>[12x]MGRILDISGQPFDFDDEMQSRSDELAMVMKRTQEHPSSGVTPNRAAQMLRDAERGDLTAQADLAFDMEEKDTHLFSELSKRRLAIQALEWRIAPARDASAQEKKDADMLNEYLHDAAWFEDALFDAGDAILKGYSMQEIEWGWLGKMRVPVALHHRDPALFCANPDNLNELRLRDASYHGLELQPFGWFMHRAKSRTGYVGTNGLVRTLIWPFIFKNYSVRDFAEFLEIYGLPMRVGKYPTGSTNREKATLMQAVMDIGRRAGGIIPMGMTLDFQSAADGQSDPFMAMIGWAEKAISKAILGGTLTTEAGDKGARSLGEVHDEVRREIRNADVGQLARSINRDLIYPLLALNSDSTIDINRLPGIVFDTSEAGDITALSDAIPKLAAGMRIPVSWIQEKLHIPQPVGDEAVFTIQPVVPDNGSQKEAALSAEDIPQEDDIDRMGVSPEDWQRSVDPLLKPVIFSVLKDGPEAAMNKAASLYPQMDDAELIDMLTRAIFVADIWGRLDAAADH;>[12x]MNYATVNDLCARYTRTRLDILTRPKTADGQPDDAVAEQALADASAFIDGYLAARFVLPLTVVPSLLKRQCCVVAWFYLNESQPTEQITATYRDTVRWLEQVRDGKTDPGVESRTAASPEGEDLVQVQSDPPVFSRKQKGFI

Myophage Mu is a representative of contractile nanomachines with a simple tail baseplate. It has the capacity to infect a range of intestinal bacteria and has extensive applications in genetic engineering research. Using cryo-EM, we resolved the three-dimensional (3D) structures of the G(+) type phage Mu in both its extended state and urea-induced contracted state, the latter lacking the baseplate, at near-atomic resolutions. The structure of extended Mu can be divided into four distinct regions: the DNA-containing head, the connector complex, the tail, and the baseplate.

Extended Mu was purified from E. coli for cryo-EM data collection, and contracted Mu was obtained by treating extended Mu samples with urea. In contrast to the extended Mu, the DNA and the TMP are ejected, and the external tail sheath contracts toward the connector complex, whereas the inner tail tube is exposed in contracted Mu. The release of the TMP and DNA in contracted Mu results in a contracted tail and an empty head. However, in both extended and contracted states, the head and the connector complex remain unchanged. Comparison of the structures of Mu in the extended and contracted states reveals that the connector complex and the tail tube remain unchanged, with the exception of the C-terminus of the tail terminator gp37, which extends to accommodate the contraction of the sheath. The Mu portal is constituted of 12 copies of the protein gp29. The Mu adaptor is constituted by 12 copies of the protein gp36, each of which comprises an α-helix domain and an elongated C-arm.> MNQIDLNVTCRYAGVFHVEKNGRY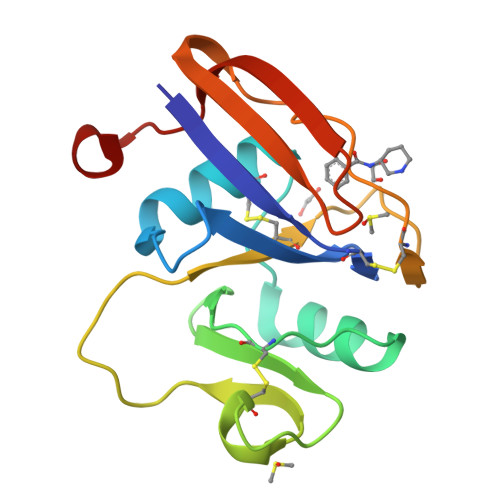SISRTEAADLCQAFNSTLPTMDQMKLALSKGFETCRYGFIEGNVVIPRIHPNAICAANHTGVYILVTSNTSHYDTYCFNASAPPEEDCTSVTDLPNSFDGPVTITIVNRDGTRYSKKGEYRTHQEDID> MLTCVTSKSIFGITTENCPDGQNL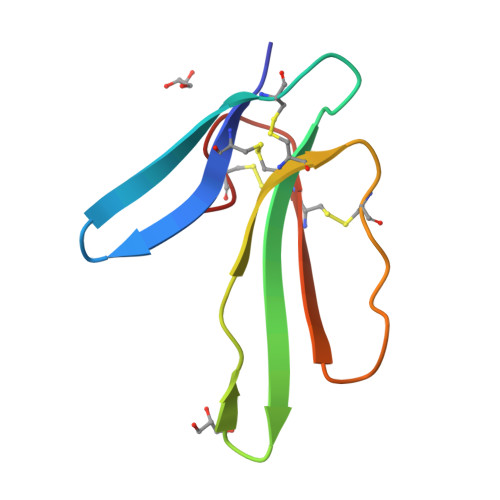CFKKWYYLNHRYSDITWGCAATCPKPTNVRETIHCCETDKCNE N-[(2S)-1-({4-[(diaminomethylidene)amino]butyl}amino)-1-oxo-3-phenylpropan-2-yl]-4-hydroxy-2-oxo-1,2-dihydroquinoline-6-carboxamide | C24 H28 N6 O4 | 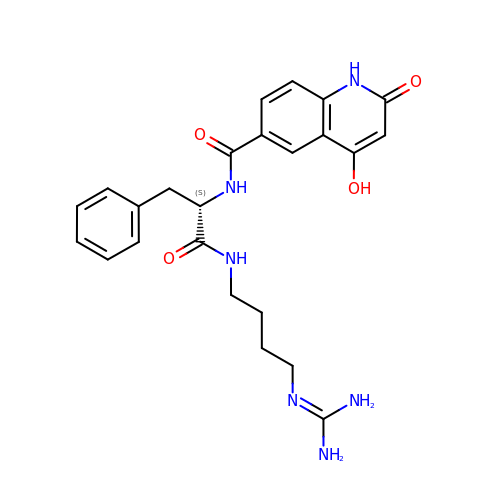DZWHLWITPPCGRM-IBGZPJMESA-N>MPPETATNPKDARHDGWQTLKRFLPYLWPADNAVLRRRVVGAILMVLLGKATTLALPFAYKKAVDAMTLGGGAQPALTVALAFVLAYALGRFSGVLFDNLRNIVFERVGQDATRHLAENVFARLHKLSLRFHLARRTGEVTKVIERGTKSIDTMLYFLLFNIAPTVIELTAVIVIFWLNFGLGLVTATILAVIAYVWTTRTITEWRTHLREKMNRLDGQALARAVDSLLNYETVKYFGAESREEARYASAARAYADAAVKSENSLGLLNIAQALIVNLLMAGAMAWTVYGWSQGKLTVGDLVFVNTYLTQLFRPLDMLGMVYRTIRQGLIDMAEMFRLIDTHIEVADVPNAPALVVNRPSVTFDNVVFGYDRDREILHGLSFEVAAGSRVAIVGPSGAGKSTIARLLFRFYDPWEGRILIDGQDIAHVTQTSLRAALGIVPQDSVLFNDTIGYNIAYGRDGASRAEVDAAAKGAAIADFIARLPQGYDTEVGERGLKLSGGEKQRVAIARTLVKNPPILLFDEACSALDTRTEQDILSTMRAVASHRTTISIAHRLSTIADSDTILVLDQGRLAEQGSHLDLL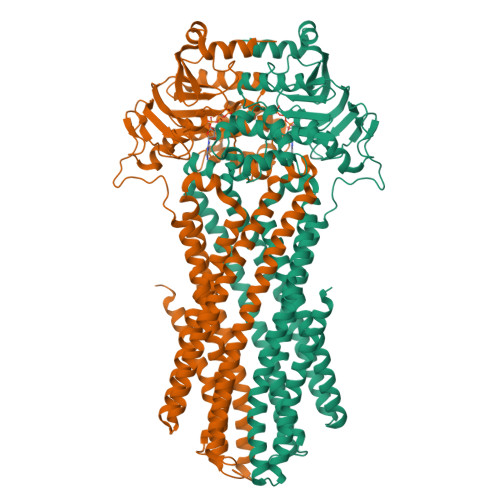RRDGLYAEMWARQAAESAEVSEAAEHHHHHH[2x]> MVPISPIETVPVKLKPGMDGPKVKQWPLTEEKIKALVEICTEMEKEGKISKIGPENPYNTPVFAIKKKDSTKWRKLVDFRE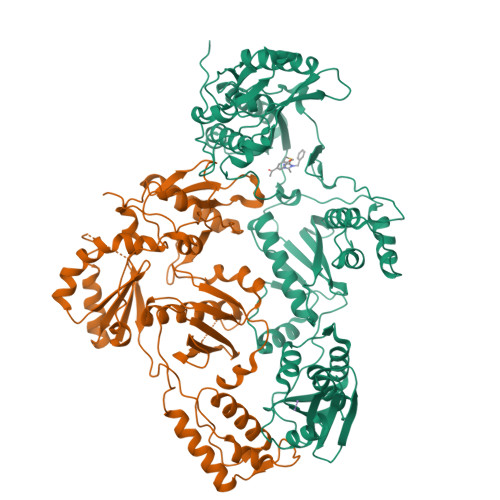LNKRTQDFWEVQLGIPHPAGLKKKKSVTVLDVGDAYFSVPLDEDFRKYTAFTIPSINNETPGIRYQYNVLPQGWKGSPAIFQSSMTKILEPFKKQNPDIVIYQYMDDLYVGSDLEIGQHRTKIEELRQHLLRWGLTTPDKKHQKEPPFLWMGYELHPDKWTVQPIVLPEKDSWTVNDIQKLVGKLNWASQIYPGIKVRQLSKLLRGTKALTEVIPLTEEAELELAENREILKEPVHGVYYDPSKDLIAEIQKQGQGQWTYQIYQEPFKNLKTGKYARMRGAHTNDVKQLTEAVQKITTESIVIWGKTPKFKLPIQKETWETWWTEYWQATWIPEWEFVNTPPLVKLWYQLEKEPIVGAETFYVDGAANRETKLGKAGYVTNKGRQKVVPLTNTTNQKTELQAIYLALQDSGLEVNIVTDSQYALGIIQAQPDKSESELVNQIIEQLIKKEKVYLAWVPAHKGIGGNEQVDKLVSAG;> GPISPIETVPVKLKPGMDGPKVKQWPLTEEKIKALVEICTEMEKEGKISKIGPENPYNTPVFAIKKKDSTKWRKLVDFRELNKRTQDFWEVQLGIPHPAGLKKKKSVTVLDVGDAYFSVPLDEDFRKYTAFTIPSINNETPGIRYQYNVLPQGWKGSPAIFQSSMTKILEPFKKQNPDIVIYQYMDDLYVGSDLEIGQHRTKIEELRQHLLRWGLTTPDKKHQKEPPFLWMGYELHPDKWTVQPIVLPEKDSWTVNDIQKLVGKLNWASQIYPGIKVRQLSKLLRGTKALTEVIPLTEEAELELAENREILKEPVHGVYYDPSKDLIAEIQKQGQGQWTYQIYQEPFKNLKTGKYARMRGAHTNDVKQLTEAVQKITTESIVIWGKTPKFKLPIQKETWETWWTEYWQATWIPEWEFVNTPPLVKLWYQ>MDHHHHHHLPNITILATGGTIAGGGDSATKSNYTTGKVGVENLVNAVPQLKDIANVKGEQVVNIGSQDMNDNVWLTLAKKINTDCDKTDGFVITHGTDTMEETAYFLDLTVKCDKPVVMVGAMRPSTSMSADGPFNLYNAVVTAADKASANRGVLVVMNDTVLDGRDVTKTNTTDVATFKSVNYGPLGYIHNGKIDYQRTPARKHTSDTPFDVSKLNELPKVGIVYNYANASDLPAKALVDAGYDGIVSAGVGNGNLYKSVFDTLATAAKTGTAVVRSSR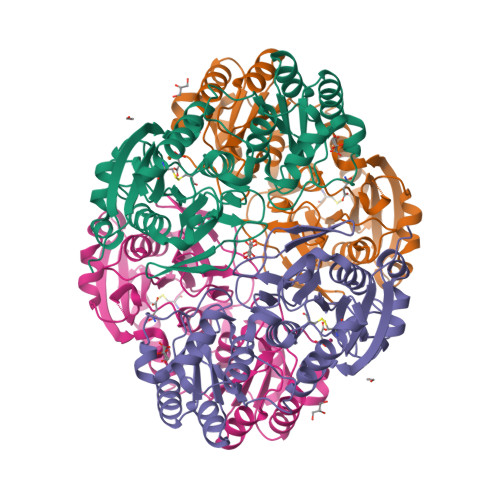VPTGATTQDAEVDDAKYGFVASGTLNPQKARVLLQLALTQTKDPQQIQQIFNQY[4x]Gabija is one of the most prevalent anti-phage defence systems, occurring in more than 15% of all sequenced bacterial and archaeal genomes, but the molecular basis of how Gabija defends cells from viral infection remains poorly understood. Bacterial Gabija defence operons encode the proteins GajA and GajB, which together protect cells against diverse phages. Gabija protein A (GajA) is a DNA endonuclease that tetramerizes to form the core of the anti-phage defence complex. Two sets of Gabija protein B (GajB) dimers dock at opposite sides of the complex and create a 4:4 GajA–GajB assembly (hereafter, GajAB) that is essential for phage resistance in vivo.

Protein interaction analysis showed that Gad1 binds directly to GajAB, and we used cryo-EM to determine a 2.6 Å structure of the GajAB–Gad1 co-complex assembly. The GajAB–Gad1 co-complex structure reveals a mechanism of inhibition in which Gad1 proteins form an oligomeric web that wraps 360° around the host defence complex. Eight copies of phage Gad1 encircle the GajAB assembly, forming a 4:4:8 GajAB–Gad1 complex that is around 775 kDa in size. Gad1 mainly recognizes the GajA nuclease core, forming extensive contacts along the surface of the GajA dimerization domain. Key GajAB–Gad1 contacts include hydrogen-bond interactions from a Gad1 positively charged loop located between β5 and β6 with GajA α2D, and hydrophobic packing interactions between Gad1 Y190 and F192 with GajA α2D. The Gad1 tetrameric interface is formed by hydrogen-bond interactions between the C-terminal ‘shoulder’ domain of each Gad1 monomer and a highly conserved set of three cysteine residues, C282, C284 and C285, which form disulfide interactions at an inter-subunit interface. The N terminus of each Gad1 monomer forms an ‘arm’ domain that extends out from the shoulder and reaches around the GajA nuclease active site to connect to a partnering Gad1 protomer from the opposite side of the complex. Each pair of Gad1 proteins that wrap around and connect at the edge of the GajAB complex are formed by one Gad1 protomer reaching out from the shoulder with an arm domain extended straight down and one Gad1 protomer reaching out with an arm domain bent around 35° to the left. Superposition of the GajAB–Gad1 and GajAB complexes shows that Gad1 binding does not induce a notable conformational change in GajAB, and suggests that Gad1 instead functions through steric hindrance of Gabija anti-phage defence. Notably, the Gad1 arm domain directly occupies this putative DNA-binding surface, supporting a model in which the phage protein directly clashes with the path of target dsDNA.

>[4x]MGSSHHHHHHGSGVKTENNDHINLKVAGQDGSVVQFKIKRHTPLSKLMKAYCERQGLSMRQIRFRFDGQPINETDTPAQLEMEDEDTIDVFQQQTGGSKFSNITIKNFRNFEKVNINLDNKNVIFGMNDIGKTNFLYALRFLLDKEIRKFGFNKSDYHKHDTSKKIEIILTLDLSNYEKDEDTKKLISVVKGARTSANADVFYIALESKYDDKELYGNIILKWGSELDNLIDIPGRGNINALDNVFKVIYINPLVDLDKLFAQNKKYIFEESQGNESDEGILNNIKSLTDQVNQQIGEMTIIKGFQQEITSEYRSLKKEEVSIELKSEMAIKGFFSDIIPYIKKDGDSNYYPTSGDGRRKMLSYSIYNYLAKKKYEDKIVIYLIEEPEISLHRSMQIALSKQLFEQSTYKYFFLSTHSPELLYEMDNTRLIRVHSTEKVVCSSHMYNVEEAYGSVKKKLNKALSSALFAERVLLIEGPSEKILFEKVLDEVEPEYELNGGFLLEVGGTYFNHYVCTLNDLGITHIIKTDNDLKSKKGKKGVYELLGLNRCLNLLGRENLDEITIDIPEDIKGKKKKERLNERKKEIFKQYKNEVGEFLGERIYLSEIDLENDLYSAIGESMKRIFENEDPVHYLQKSKLFNMVELVNNLSTKDCFDVFEHEKFACLKELVGSDRG;>MSREQIIKDGGNILVTAGAGSGKTTILVSKIEADLKENKTHYSIAAVTFTNKAAKEIEGRLGYSSRGNFIGTNDGFVESEIIRPFIKDAFGNDYPDNFTAEYFDNQFASYDKGLQVLKYQNILGTYSNPKKNFKFQLALDILKKSLVARQYIFSKYFKIFIDEYQDSDKDMHNLFMYLKDQLKIKLFIVGDPKQSIYIWRGAEPENFNGLIENSTDFNKYHLTSNFRCCQDIQNYSNLFNEETRSLIKEKNEVQNVISIADDMPISDILLKLTEEKQVLNIEAELVILVRRRNQAIEIMKELNEEGFNFIFIPQTPLDRATPNATLLKEVIKYVKNDRYSIYDLAAEIVGNLSSREIKEIQKIINELLVPNINQVLINQVLINLFAKLEITLDTREITAFTEVMMTNEFDIAFDTNEYLHKIFTVHSAKGLEFNQVIITASDYNVHYNRDTNEHYVATTRAKDKLIVIMDNKKYSDYIETLMKELKIKNIIKSI[4x];>[8x]MKLIGIKTSNCFLVSDNIEGKRYFHSQLDELLFDGKRATETYKSDWFKLEKEPSVIEKQMPAKKINHRYELKEGFQESELTPKVIKASYIGEDSEYYEVKGLYDLKFEEIPQQNEKIEFEMNVIEEIDGELKLQSHNFNLNYNLLDRIQTHPMLLETKPCYLSQEESYKIIRNHIKANINPKFARITSDYDFCLTVVKVLELYKPHEYIVDLNAMYKRRKPKLEKRFQTKREVEIYKVAPKAYQSYPIVEPFSGKDVEDLKSNIKKFLDDLMAKINEPLVECKCCKGRGVILNEN N-cyclohexyl-4-(1H-imidazol-5-yl)piperidine-1-carbothioamide 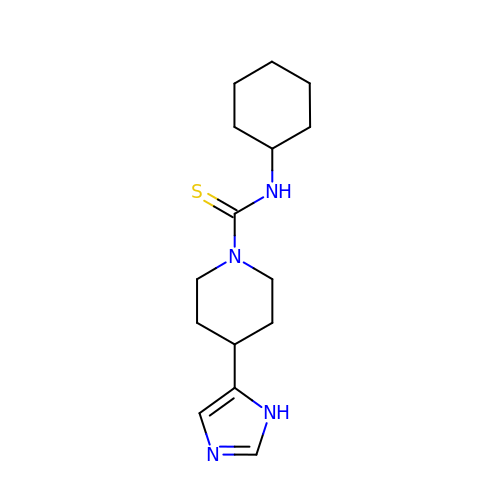| C15 H24 N4 S | QKDDJDBFONZGBW-UHFFFAOYSA-N> GSHMKNSVSVDLPGSMKVLVSKSSNADGKYDLIATVDALELSGTSDKNNGSGVLEGVKADASKVKLTISDDLGQTTL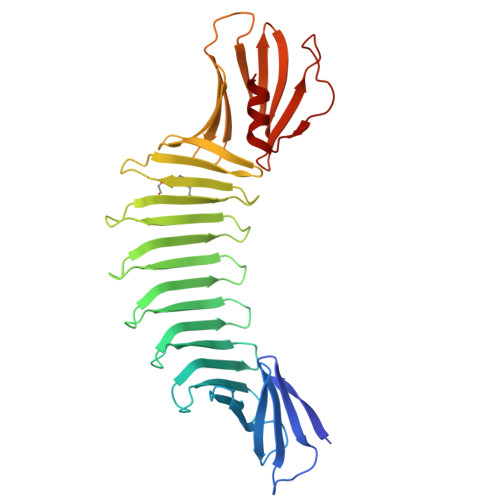EVFKSDGSTLVSKKVTSKDKSSTEEKFNEKGELSEKKITRADKSSTEEKFNEKGELSEKKITRADKSSTEEKFNEKGELSEKKITRADKSSTEEKFNEKGEVSEKIITRADGTRLEYTGIKSDGSGKAKEVLKGYVLEGTLTAEKTTLVVKEGTVTLSKNISKSGEVSVELNDTDSSAATKKTAAWNSGTSTLTITVNSKKTKDLVFTSSNTITVQQYDSNGTSLEGSAVEITKLDEIKNALK>[6x]LPNITILATGGTIAGGGDSATKSNYTVGKVGVENLVNAVPQLKDIANVKGEQVVNIGSQDMNDNVWLTLAKKINTDCDKTDGFVITHGTETMEETAYFLDLTVKCDKPVVMVGAMRPSTSMSADGPFNLYNAVVTAADKASANRGVLVVMNDTVLDGRDVTKTNTTDVATFKSVNYGPLGYIHNGKIDYQRTPARKHTSDTPFDVSKLNELPKVGIVYNYAN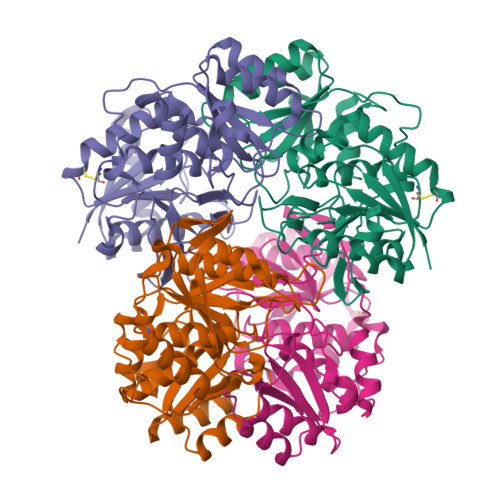ASDLPAKALVDAGYDGIVSAGVGNGNLYKSVFDTLATAAKTGTAVVRSSRVPTGATTQDAEVDDAKYGFVASGTLNPQKARVLLQLALTQTKDPQQIQQIFNQY> MLCVDVNVLVYAHRADLREHADYRGLLERLANDDEPLGLPDSVLAGFIRVVTNRRVFTEPTSPQDAWQAVDALLAAPAAMRLRPGERHWMAFRQLASDVDANGNDI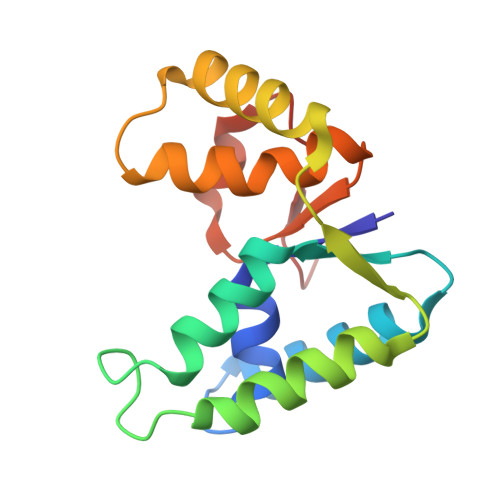ADAHLAAYALENNATWLSADRGFARFRRLRWRHPLD>[2x]MRGSHHHHHHGSASFLKKTMPFKTTIEGTV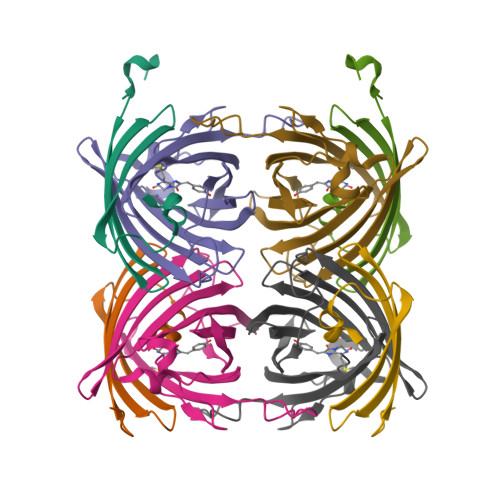NGHYFKCTGKGEGNPFEGTQEMKIEVIEGGPLPFAFHILSTSC;>[2x]MYGSKTFIKYVSGIPDYFKQSFPEGFTWERTTTYEDGGFLTAHQDTSLDGDCLVYKVKILGNNFPADGPVMQNKAGRWEPATEIVYEVDGVLRGQSLMALKCPGGRHLTCHLHTTYRSKKPASALKMPGFHFEDHRIEIMEEVEKGKCYKQYEAAVGRYCDAAPSKLGHN>MDYKDDDDKENLYFQGMNGEAICSALPTIPYHKLADLRYLSRGASGTVSSARHADWRVQVAVKHLHIHTPLLDSERKDVLREAEILHKARFSYILPILGICNEPEFLGIVTEYMPNGSLNELLHRKTEYPDVAWPLRFRILHEIALGVNYLHNMTPPLLHHDLKTQNILLDNEFHVKIADFGLSKWRMMSLSQSRSSKSAPEGGTIIYMPPENYEPGQKSRASIKHDIYSYAVITWEVLSRKQPFEDVTNPLQIMYSVSQG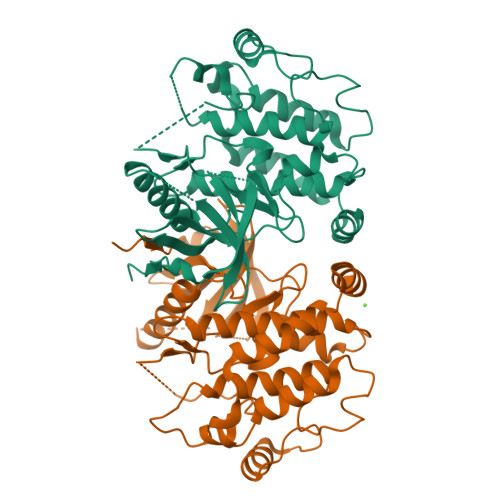HRPVINEESLPYDIPHRARMISLIESGWAQNPDERPSFLKCLIELEPVLRTFEEITFLEAVIQLK[2x]> GHMNNLARLEPEVLSRHAISSEQLGIWYIQRLEPTCSAYNMVVAFDVKVNQSLGNKPIEILEAVMHDYPLLRVSMPANDQGIEQLIWDRVYPNIIFSDARHIEASDLTQLVEQDTKQPFDLTQPPLWRIHCYECGQNHYVIAFVIHHALMDFWSIGLLLRDVSKRFGLVAESDAVNGIEFVQYADKQQSSVIDDTDESLIFWKNALKHAPHVHSIPLDYPRPAVQQHKGSSLVFRVSESVSSGLVNLAKDYEITLFGLVLSGFYVLLHKLSNENNLVIATPVAGRLERSLRNALGQFVNTIAIHMDIDADQTLRQFTQQVQEQLRQSLKHQKIAFSRVVEAVSPKRDGSINPLAQIGMFWERLGGMDEFKELLLPIQTPATLVGQDLTLGSFPVRQQEGQLDITLEMGGEYQGELVGVLKYNTDLFSAQSAENMVQLLQAVLSEMVAHPERKIVELDIAPDYKDGIQFEALRGKATDYAQHDLFAMILKQIDERGDNHALTSNDHTVSYRELGQHIAGIAEYLRAHGITQGDRVGLMLDRTALLPAAILGIWAAGAAYVPLDPNFPTERLQNIIEDAEPKVILTQTELMDGLNVSVPRLDINQAGVVALEQVRETLAFGDIAYVMYTSGSTGKPKGVRIGHPSIINFLLSMNDRLQVTTETQLLAITTYAFDISILELLIPLM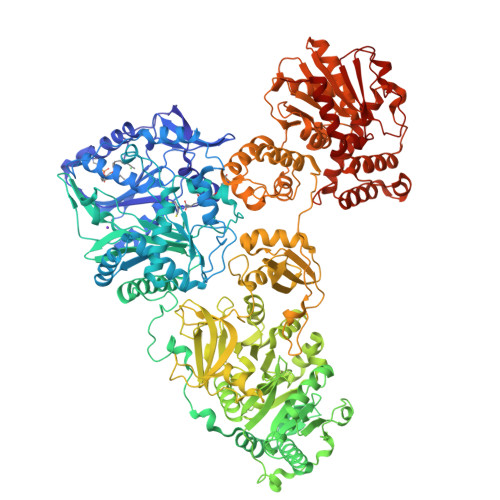YGGVVHVCPREVSQDGIQLVDYLNAKSINVLQATPATWKMLLDSEWSGNAGLTALCGGEALDTILAEKLLGKVGCLWNVYGPTETTVWSSAARITDAKYIDLGEPLANTQLYVLDEQQRLVPPGVMGELWIGGDGLAVDYWQRPELTDAQFRTLPSLPNAGRLYRTGDKVCLRTDGRLTHHGRLDFQVKIRGFRIELGEIENVLKQIDGITDAVVLVKTTGDNDQKLVAYVTGQELDIAGLKKNLQIHLPAYMVPSAFIRLDEFPMTANKKLDRKAFPEPIFEQSNDYVAPRDPIEIELCTTFEQILSVKRVGIHDDFFELGGHSLLAVKLVNHLKKAFGTELSVALLAQYSTVERLGEIIRENKEIKPSIVIELRRGTYEQPLWLFHPIGGSTFCYMELSRHLNPNRTLRAIQSPGLIEADAAEVAIEEMATLYIAEMQKMQPQGPYFLGGWCFGGAIAYEISRQLRQMGQQVTGIVMIDTRAPIPENVPEDADDAMLLSWFARDLAAPYGKKLTIPAQYLRELSPDQMFDHVLKEAKAINVLPLDADPSDFRLYFDTYLANGIALQTYFPEPEDFPILLVKAKDEQEDFGESLGWDQLVKDTLTQVDLPGDHSSIMYAENVVAVAQTIDQMYPIP> EVKQENRLLNESESSSQGLLGYYFSDLNFQAPMVVTSSTTGDLSIPSSELENIPSENQYFQSAIWSGFIKVKKSDEYTFATSADNHVTMWVDDQEVINKASNSNKIRLEKGRLYQIKIQYQRENPTEKGLDFKLYWTDSQNKKEVISSDNLQLPELKQKSSNSRKKRSTSAGPTVPDRDNDGIPDSLEVEGYTVDVKNKRTFLSPWISNIHEKKGLTKYKSSPEKWSTASDPYSDFEKVTGRIDKNVSPEARHPLVAAYPIVHVDMENIILSKNEDQSTQNTDSETRTISKNTSTSRTHTSEVHGNAEVHASFFDIGGSVSAGFSNSNSSTVAIDHSLSLAGERTWAETMGLNTADTARLNANIRYVNTGTAPIYNVLPTTSLVLGKNQTLATIKAKENQLSQILAPNNYYPSKNLAPIALNAQDDFSSTPITMNYNQFLELEKTKQLRLDTDQVYGNIATYNFENGRVRVDTGSNWSEVLPQIQETTARIIFNGKDLNLVERRIAAVNPSDPLETTKPDMTLKEALKIAFGFNEPNGNLQYQGKDITEFDFNFDQQTSQNIKNQLAELNATNIYTVLDKIKLNAKMNILIRDKRFHYDRNNIAVGADESVVKEAHREVINSSTEGLLLNIDKDIRKILSGYIVEIEDTEGLKEVINDRYDMLNISSLRQDGKTFIDFKKYNDKLPLYISNPNYKVNVYAVTKENTIINPSENGDTSTNGIK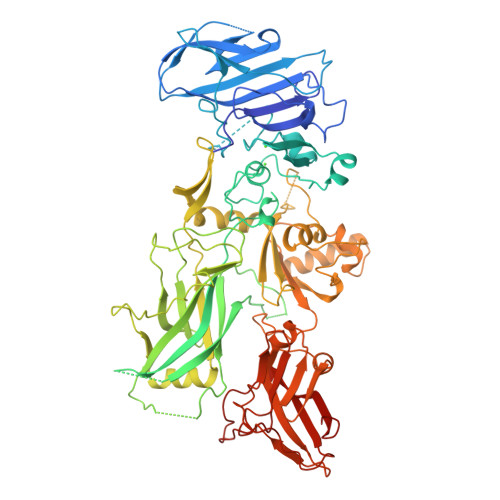KILIFSKKGYEIG Within the protein lysine methyltransferase (PKMT) family of enzymes, one branch contains five enzymes that share two highly conserved, functional domains: the catalytic SET domain and the MYND domain; these five enzymes are known as SMYD1, SMYD2, SMYD3, SMYD4 and SMYD5. Among the SMYD enzymes, SMYD2 and SMYD3 have been implicated as targets for a variety of cancer indications. In the current study we exemplify pharmacophore series for SMYD2 and SMYD3 that show low nanomolar potency against their targets and significant selectivity over all other enzymes tested with favorable physicochemical properties and pharmacological tractability. S2 Table Crystallographic data collection and refinement statistics for SMYD2 and SMYD3 crystal structures.

Structure-activity relationship studies of SMYD3 inhibitors led to the isoxazole sulfonamide series exemplified by EPZ028862, another molecule displaying similarly potency against SMYD3 in biochemical and cellular assays with physicochemical properties suitable for in vivo studies. In addition, EPZ028862 was tested against a panel of 15 methyltransferase enzymes to check the selectivity of the compound for SMYD3. For all enzymes tested, including the closely related enzyme SMYD2, no inhibition was seen up to 10 μM. EPZ028862 inhibition is best described as noncompetitive versus MEKK2 (Eq 6) and mixed-type inhibition versus SAM (Eq 5). Kinetic constants kon (6.1 ± 1.1 x 105 M-1s-1) and koff, (2.1 ± 0.57 x 10−4 s-1) were based on fitted values from seven replicate measurements (mean ± standard deviation). Therefore, in order to provide support that EPZ028862 binds endogenous SMYD3 rather than only the overexpressed protein, a cellular thermal shift assay (CETSA) was performed that reported a 1.4 μM EC50 for SMYD3 binding and verified target engagement of EPZ028862 for endogenous SMYD3. SMYD3 has also been shown to regulate MAPK pathways by methylating MAP3K2. Instead, cell activity of SMYD3 was determined using a previously documented engineered system in which both SMYD3 and MAP3K2 were cotransfected into 293T cells and inhibition of Lys260 methylation of MAP3K2 was measured. Treatment of NSCLC and other lung cancer cell lines with and without KRAS mutations at concentrations as high as 25 µM had no impact on proliferation. We subsequently extended these studies to a broad panel of 240 cancer cell lines (Eurofins Panlabs Oncopanel) across a variety of indications; again, no proliferative IC50 was observed for this compound in any of the cancer cell lines at concentrations as high as 25 µM.

> MEPLKVEKFATANRGNGLRAVTPLRPGELLFRSDPLAYTVCKGSRGVVCDRCLLGKEKLMRCSQCRVAKYCSAKCQKKAWPDHKRECKCLKSCKPRYPPDSVRLLGRVVFKLMDGAPSESEKLYSFYDLESNINKLTEDKKEGLRQLVMTFQHFMREEIQDASQLPPAFDLFEAFAKVICNSFTICNAEMQEVGVGLYPSISLLNHSCDPNCSIVFNGPHLLLRAVRDIEVGEELTICYLDMLMTSEERRKQLRDQYCFECDCFRCQTQDKDADMLTGDEQVWKEVQESLKKIEELKAHWKWEQVLAMCQAIISSNSERLPDINIYQLKVLDCAMDACINLGLLEEALFYGTRTMEPYRIFFPGSHPVRGVQVMKVGKLQLHQGMFPQAMKNLRLAFDIMRVTHGREHSLIEDLILLLEECDANIRAS(1~{S},10~{S})-12-cyclobutyl-5-methyl-1-oxidanyl-10-propan-2-yl-9,12-diazatricyclo[8.2.1.0^{2,7}]trideca-2(7),3,5-trien-11-one | C19 H26 N2 O2 | 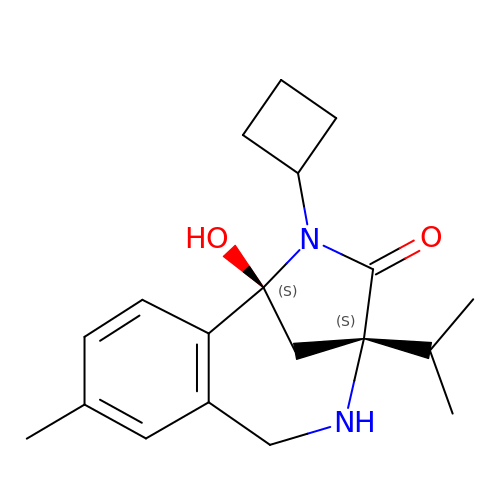HABACEYDTYGRSK-OALUTQOASA-N> MTTLEAFAKARSEGRAA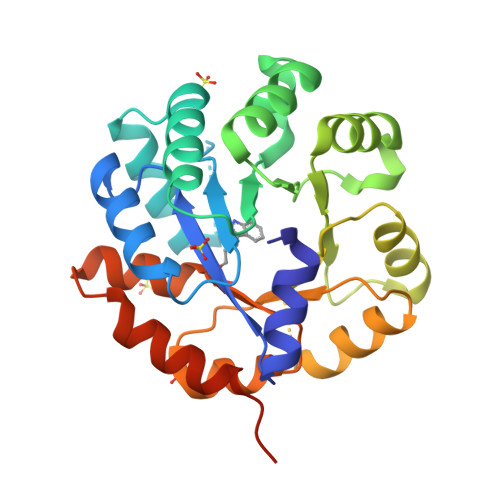LIPYLTAGFPSREGFLQAVEEVLPYADLLEIGLPYSDPLGDGPVIQRASELALRKGMSVQGALELVREVRALTEKPLFLMTYLNPVLAWGPERFFGLFKQAGATGVILPDLPPDEDPGLVRLAQEIGLETVFLLAPTSTDARIATVVRHATGFVYAVSVTGVTGMRERLPEEVKDLVRRIKARTALPVAVGFGVSGKATAAQAAVADGVVVGSALVRALEEGRSLAPLLQEIRQGLQRLEANPGLKESSKKPLP6-(3,4-dimethylphenyl)-3-[[4-[3-(4-methylpiperazin-1-yl)propoxy]phenyl]amino]pyrazine-2-carboxamide | C27 H34 N6 O2 | 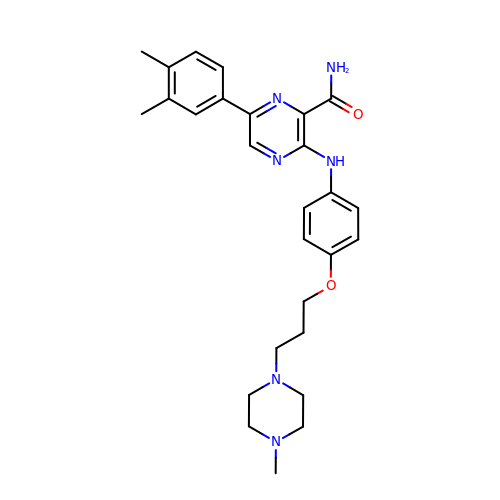SMJHCUSNBTWDKM-UHFFFAOYSA-N> MKKLILLTLIIASFDIYAIDFVYRVDPNPPDVIFRDGFSLLGYNRDLQQLISGRSCAGGSSDSRYIVTTSDINKTYAIARAYYSHSKFKGNLYRYKIRADNNFYSLTPSVNYLESQGGHFNAYEKSMIRLQSEYVSTLSILPENIQKAVALVYDSSTGQIKDGTSTINTDYVSISSVSNPGVIPFLPEPQANTQQRIDAFGSLISSCFSIYSVCQTHRGQKTEVYKMPFYDARPVIQFIISGN;>[5x]MKKITSVCALLSLICSFNASAEWTGDYENIGYFSHEVISEFHVGQIDGGAYFCIKAVKADGSRSTPLIACSVSNESVWAPSFKVLLEQARYFYVTEQSVRIYYDHNVWTNQPFVNTFSTNALVGLSSCSAATDCFGPGKPKSKSKRDVEQ

In this study, we identified and characterized a typhoid toxin-like A2B5 toxin, designated diarizonae toxin (DiaT), as a key virulence factor in Salmonella diarizonae. The DiaT genomic islet encodes two distinct B subunits, PltBd1 and PltBd2, which exhibit unique functional roles. Through genetic and functional analyses, we demonstrate that the heteropentameric assembly of PltBd1 and PltBd2 is essential for cytotoxicity, with our data suggesting PltBd1 facilitates toxin secretion and PltBd2 mediates host cell targeting. The holotoxin consists of a pentameric B subunit arrangement supporting a single PltA subunit, with the amphipathic C-terminal tail of PltA extending into the central pore formed by the B subunits.

To validate the structural insights from the cryo-EM map of the endogenously expressed DiaT holotoxin, we recombinantly expressed PltBd1 homopentameric holotoxin, PltBd2 homopentameric holotoxin, and PltBd1/PltBd2 heteropentameric holotoxin in E. coli. Cryo-EM analysis resolved these structures at resolutions of 3.05 Å, 2.61 Å, and 2.94 Å, respectively. A localized distortion in the central pore was observed near Tyr70 in PltBd1, where the bulky phenolic side chain creates steric hindrance, causing contraction at this site. Pore radius measurements confirmed that the PltBd1 homopentamer exhibits the smallest pore radius with significant distortion, while the PltBd2 homopentamer displays a larger and straighter pore. Further analysis of PltA’s interactions with distinct B subunits identified a critical hydrophobic interaction between Ile227 of PltA and Ile71 of PltBd2. This interaction is weaker in the PltBd1 homopentamer due to the shorter side chain of Val73 in PltBd1. All holotoxins demonstrated cytotoxic activity, but the PltBd2 homopentamer exhibited the highest potency, approximately threefold greater than the PltBd1/PltBd2 heteropentameric toxin (DiaT) and nearly 75-fold greater than the PltBd1 homopentamer. Individual complementation with either pltBd1 or pltBd2 led to the assembly of holotoxins with homopentameric B subunits, yet neither restored the cytotoxicity of S. diarizonae. However, only PltBd1 displayed substantial binding to Neu5Gc-terminated glycans.>[2x]MTIICSVDIGIKNPAYTIFRYEDSKVSLIAIEKSDW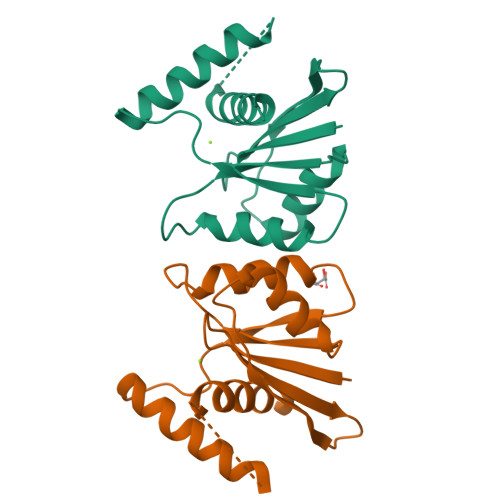SDNWEYNVTKDLTKYNPDIIVLEKQGYRSPNAKIIYFIKGFFYNTNTSVIVRNPTFQGGSYSDRKKQSVITFMDKLSRYSDHIDDILSSFTKLDDIADSFNLGIAYIESTFKKNVK>[2x]MKDRTQELRTAKDSDDDDDVTVTVDRDRFMDEFFEQVEEIRGFIDKIAENVEEVKRKHSAILASPNPDEKTKEELEELMSDIKKTANKVRSKLKSIEQSIEQEEGLNRSSADLRIRKTQHSTLSRKFVEVMSEYNATQSDYRERCKGRIQRQLEITGRTTTSEELEDMLESGNPAIFASGIIMDSSISKQALSEIETRHSEIIKLENSIRELHDMFMDMAMLVESQGEMIDRIEYNVEHAVDYVERAVSDTKKAVKYQSKARRKKIM;> MGSSHHHHHHSQDPNSMAEDADMRNELEEMQRRADQLADESLESTRRMLQLVEESKDA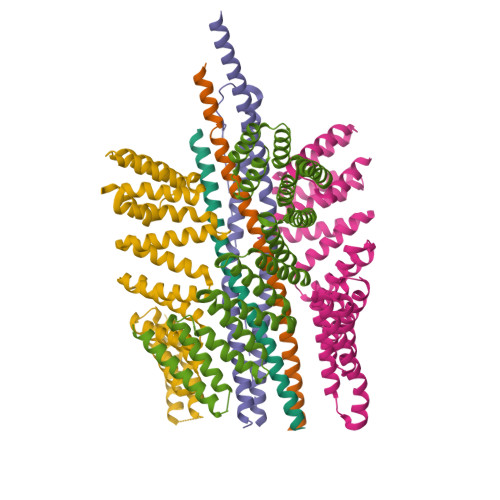GIRTLVMLDEQGEQLERIEEGMDQINKDMKEAEKNLTDLGKFAGLAVAPANKLKSSDAYKKAWGNNQDGVVASQPARVVDEREQMAISGGFIRRVTNDARENEMDENLEQVSGIIGNLRHMALDMGNEIDTQNRQIDRIMEKADSNKTRIDEANQRATKMLGSG;>GMDTSGKQAEAMALLAEAERKVKNSQSFFSGLFGGSSKIEEACEIYARAANMFKMAKNWSAAGNAFCQAAQLHLQLQSKHDAATCFVDAGNAFKKADPQEAINCLMRAIEIYTDMGRFTIAAKHHISIAEIYETELVDVEKAIAHYEQSADYYKGEESNSSANKCLLKVAGYAAQLEQYQKAIDIYEQVGTSAMDSPLLKYSAKDYFFKAALCHFCIDMLNAKLAVQKYEELFPAFSDSRECKLMKKLLEAHEEQNVDSYTESVKEYDSISRLDQWLTTMLLRIKKTIQGDEEDLR[3x]> GSPGISGGGGGILDSMDVVSLDKPFMYFEEIDNELDYEPESANEVAKKLPYQGQLKLLLGELF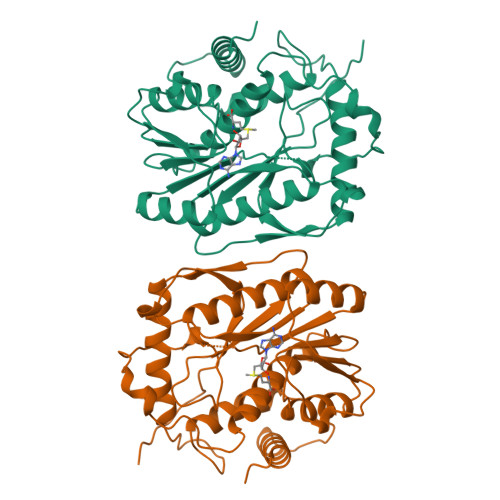FLSKLQRHGILDGATVVYIGSAPGTHIRYLRDHFYNLGVIIKWMLIDGRHHDPILNGLRDVTLVTRFVDEEYLRSIKKQLHPSKIILISDVASAAGGNEPSTADLLSNYALQNVMISILNPVASSLKWRCPFPDQWIKDFYIPHGNKMLQPFAPSYSAEMRLLSIYTGENMRLTRVTKSDAVNYEKKMYYLNKIVRNKVVVNFDYPNQEYDYFHMYFMLRTVYCNKTFPTTKAKVLFLQQSIFRFLNIPTTSTEKVSHEPIQRKISSKNSMSKNRNSKRSVRSNK> MMEYEDLELITIWPSPTKNKLCQFIKQNLSKEHVVTQLFFIDATSSFPLSQFQKLVPPTLPENVRIYENIRINTCLDLEELSAITVKLLQILSMNKINAQRGTEDAVTEPLK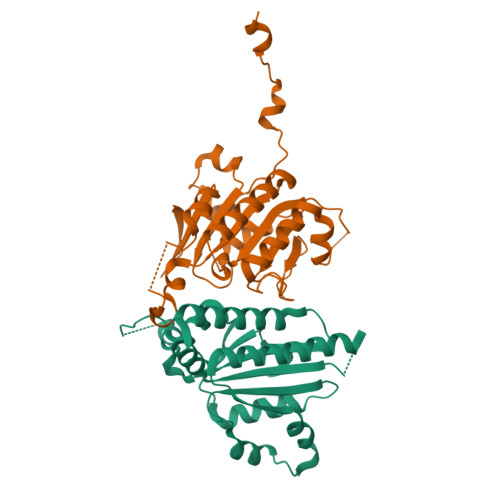IILYINGLEVMFRNSQFKSSPQRSHELLRDTLLKLRVMGNDENENASIRTLLEFPKEQLLDYYLKKNNNTRTSSVRSKRRRIKNGDSLAEYIWKYYADSLFE;> MGSSHHHHHHSHGSMEVLKNIRIYPLSNFITSTKNYINLPNELRNLISEEQESKLGFLHIIESDFKPSVALQKLVNCTTGDEKILIIDIVSIWSQQKQRQHGAIYMNSLSCINITGLIVFLELLYDSPMDALRRCQVDNFNFQLRGIVIDNLSFLNFESDKNYDVINLSKFEKLFKILRKLREFLGCWIITKSFPTDFYNGIENTLVDKWSIKRKSGVTLYPTKLPDSYMKGMDLIIYREVVDGRPQYRRIAALEE>MTINVNTNVSAMTAQRYLTKATGELNTSMERLSSGNRINSAKDDAAGLQISNRLTAQSRGLDVAMRNANDGISIAQTAEGAMNESTSILQRMRDLALQSANGTNSASERQALNEESVALQDELNRIAETTSFGGRKLLNGSFGEASFQIGSSSGEAIIMGLTSVRADDFRMGGQSFIAEQPKTKEWGVPPTARDLKFEFTKKDGEAVVLDIIAKDGDDIEELATYINGQTDLFKASVDQEGKLQIFVAEPNIEGNFN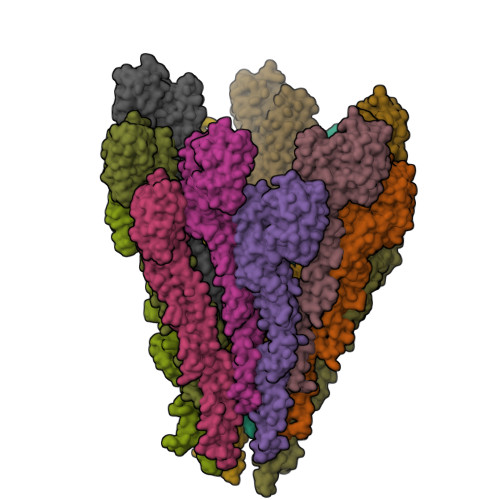ISGGLATELGLNGGPGVKTTVQDIDITSVGGSQNAVGIIDAALKYVDSQRADLGAKQNRLSHSISNLSNIQENVEASKSRIKDTDFAKETTQLTKSQILQQAGTSILAQAKQLPNSAISLLQ[14x]>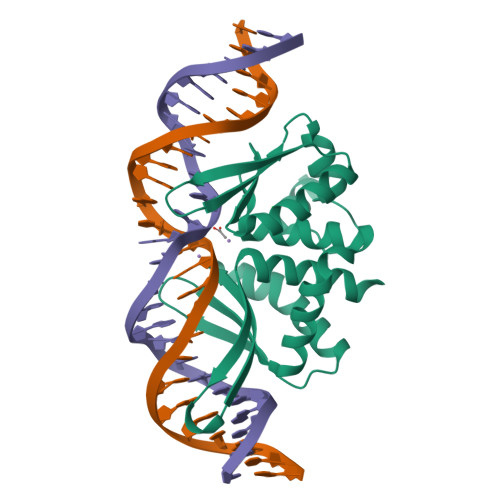[3x]AHNNENVSGISAYLLGLIIGDGGLYKLKYKGNRSEYRVVITQKSENLIKQHIAPLMQFLIDELNVKSKIQIVKGDTRYELRVSSKKLYYYFANMLERIRLFNMREQIAFIKGLYVAAGDKTLKRLRIWNKNKALLEIVSRWLNNLGVRNTIHLDDHRHGVYVLNISLRDRIKFVHTILSSHLNPLPPEAAALEHHHHHH>[2x]MDWGRFVEEKVREIRETVGDSKAIIALSGGVDSSTAAVLAHKAIGDRLHAVFVNTGFLRKGEPEFVVKTFRDEFGMNLHYVDAQDRFFSALKGVTDPEEKRKIIGRVFIEVFEEVAKKIGAEYLIQGTIAPDWIESQGKIKSHHNVGGLPEKLNLKLIEPLRDLYKDEVRELAKFLGLPEKIYN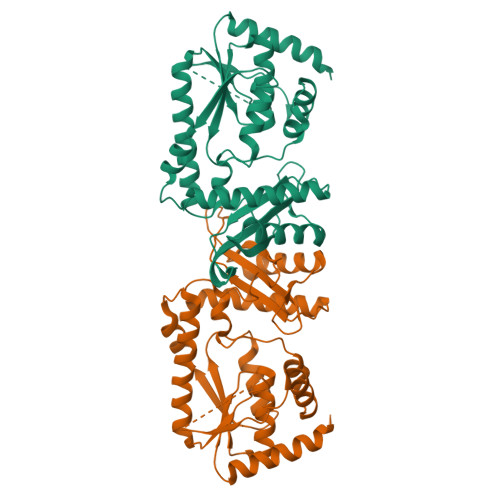RMPFPGPGLAVRVIGEVTPEKIRIVREANAIVEEEVERAGLRPWQAFAVLLGVKTVGVQGDIRAYKETIAVRIVESIDGMTANAMNVPWEVLQRIAFRITSEIPEVGRVLYDITNKPPATIEFE>SKGKLPPVYPVTVPILGHIIQFGKSPLGFMQECKRQLKSGIFTINIVGKRVTIVGDPHEHSRFFLPRNEVLSPREVYSFMVPVFGEGVAYAAPYPRMREQLNFLAEELTIAKFQNFVPAIQHEVRKFMAANWDKDEGEINLLEDCSTMIINTACQCLFGEDLRKRLDARRFAQLLAKMESSLIPAAVFLPILLKLPLPQSARCHEARTELQKILSEIIIARKEEEVNKDSSTSDLLSGLLSAVYRDGTPMSLHEVCGMIVAAMFAGQHTSSITTTWSMLHLMHPANVKHLEALRKEIEEFPAQLNYNNVMDEMPFAERCARESIRRDPPLLMLMRKVMADVKVGS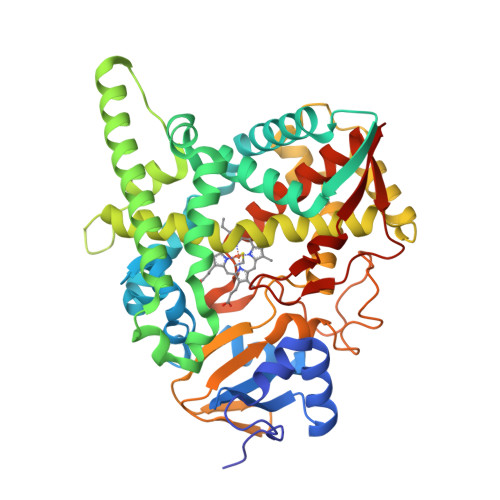YVVPKGDIIACSPLLSHHDEEAFPEPRRWDPERDEKVEGAFIGFGAGVHKCIGQKFGLLQVKTILATAFRSYDFQLLRDEVPDPDYHTMVVGPTASQCRVKYIRR[4x]> AVRGSII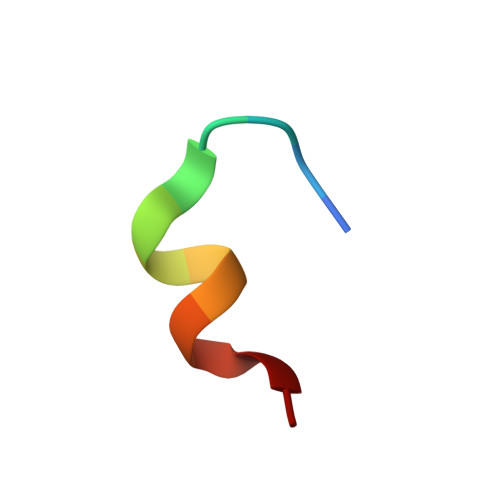ANMLQE>[24x]MKTINSVDTKEFLNHQVANLNVFTVKIHQIHWYMRGHNFFTLGEKMDDLYSEFGEQMDEVAERLL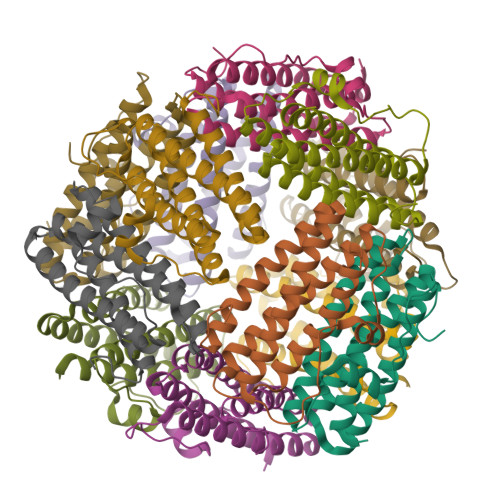AIGGSPFSTLKEFLENASVEEAPYTKPKTMDQLMEDLVGTLELLRDEYKQGIELTDKEGDDVTNDMLIAFKASIDKHIWMFKAFLGKAPLE> 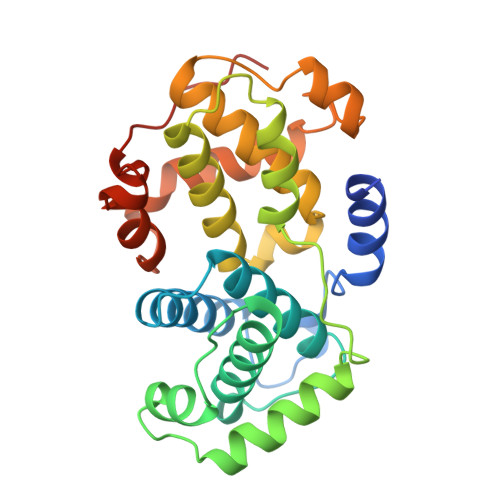GVNEVPDYHEDIHTYLREMEVKCKPKVGYMKKQPDITNSMRAILVDWLVEVGEEYKLQNETLHLAVNYIDRFLSSMSVLRGKLQLVGTAAMLLASKFEEIYPPEVAEFVYITDDTYTKKQVLRMEHLVLKVLAFDLAAPTINQFLTQYFLHQQPANCKVESLAMFLGELSLIDADPYLKYLPSVIAAAAFHLALYTVTGQSWPESLVQKTGYTLETLKPCLLDLHQTYLRAPQHAQQSIREKYKNSKYHGVSLLNPPETLNLHHHHHH> MKNVYLPITVDHIARVEGKGGVEIVVGDDGVKEVKLNIIEGPRFFEAITLGKKLDEALAIYPRICSFCSAAHKLTAVEAAEKAIGFTPREEIQALREVLYIGDMIESHALHLYLLVLPDYLGYSGPLHMIDEYKKEMSIALDLKNLGSWMMDELGSRAIHQENAVLGGFGKLPDKSVLENMKRRLKEALPKAEYTFELFTKLEQYEEVEGPITHIAVKPRNGVYGIYGDYLKASDGNEFPSEEYREHIKEFVVEHSFAKHSHYHGKPFMVGAISRLVNNADTLYGRAKELYESYKDLLRSTNPFANNLAQALELVYFTERAIDLIDEALAKWPIRPRDEVALKDGFGVSTTEAPRGVLVYALKVENGRVSYADIITPTAFNLAMMEQHVRMMAEKHYNDDPEKLKLLAEMVV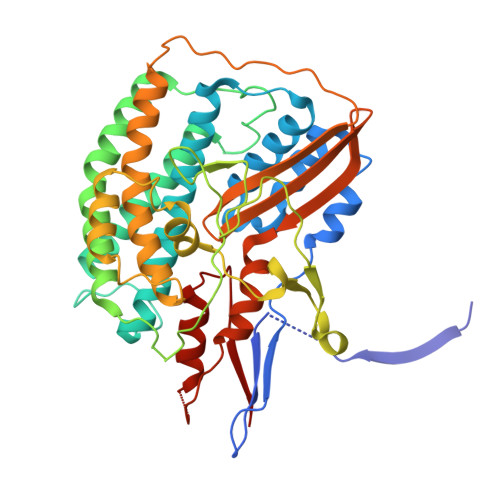RAYDPCISCSVHVARL>GMSENSSVRHGLTSAQHCVWLAQQLDPRGAHYRTGSCLEIDGPLDHAVLSRALRLTVAGTETLCSRFLTDEEGRPYRAYCPPAPEGSAAVEDPDGVPYTPVLLRHIDLSGHEDPEGEAQRWMDRDRATPLPLDRPGLSSHALFTLGGGRHLYYLGVHHIVIDGTSMALFYERLAEVYRALRDGRAVPAAAFGDTDRMVAGEEAYRASARYERDRAYWTGLFTDRPEPVSLTGRGGGRALAPTVRSLGLPPERTEVLGRAAEATGAHWARVVIAGVAAFLHRTTGARDVVVSVPVTGRYGANARITPGMVSNRLPLRLAVRPGESFARVVETVSEAMSGLLAHSRFRGEDLDRELGGAGVSGPTVNVMPYIRPVDFGGPVGLMRSISSGPTTDLNIVLTGTPESGLRVDFEGNPQVYGGQDLTVLQERFVRFLAELAADPAA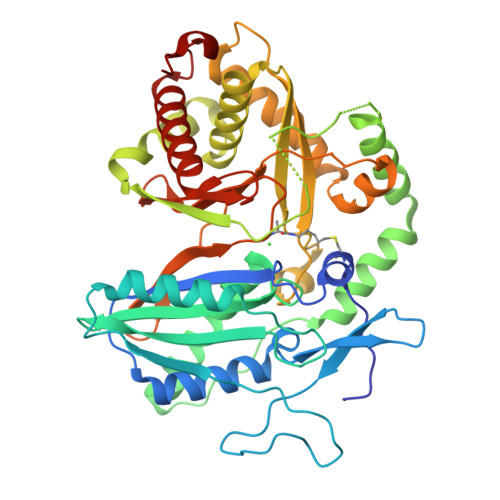TVDEVALLT[2x]>[2x]GPMDYYTLLGVDKGCSEDDLRRAYLKLAMKWHPDKHVNKGSKVEAEEKFKNICEAYSVLSDNEKRVKYDL

In the Laverania subgenus of malaria parasites, of which P. falciparum is the only human-infective member, a single Hsp70 chaperone, Hsp70-x, is exported to the host cell. Common to all Laverania parasites is an expanded set of exported proteins for host cell remodeling; thus, it is believed that Hsp70-x ensures the correct folding of these proteins, thereby supporting parasite survival and virulence functions. In addition to PfEMP1 and PfHsp70-x, J-dots contain multiple Hsp40 (also known as DnaJ) cochaperone proteins, which can stimulate Hsp70 activity. At least one of these cochaperones, PFA0660w (pf3d7_0113700), was shown to preferentially stimulate PfHsp70-x activity compared with a human Hsp70 (19).

Consistent with previous studies using full-length PFA0660w, the J-domain of this protein (PFA0660wJ) stimulated PfHsp70-x activity by ∼2-fold. We sought to investigate the structural basis of PfHsp70-x and Hsc70 stimulation by parasite cochaperones, focusing particularly on PFA0660w whose expression coincides with large-scale erythrocyte remodeling. To that end, we resolved the crystallographic structure of PFA0660wJ at 1.38 Å resolution and assigned the NMR spectra of PFA0660wJ in a sequence-specific manner. This allowed us to study the physical interaction of PFA0660wJ with PfHsp70-x or Hsc70 at amino acid–level resolution. As anticipated from the chaperone stimulation assays above, both PfHsp70-x and Hsc70 interacted directly with PFA0660wJ, as evidenced by changes in the intensity of [15N]-labeled PFA0660wJ NMR peaks corresponding to specific amino acids upon titration of this protein with unlabeled PfHsp70-x or Hsc70. Furthermore, we noted that PfHsp70-x produced larger changes in NMR peak intensity compared with Hsc70, suggesting that the PfHsp70-x–PFA0660wJ interaction is stronger than that between PFA0660wJ and the human chaperone, which is consistent with the biochemical assays above. To evaluate whether these interactions are compatible with the formation of canonical chaperone-cochaperone complexes, we mapped the PFA0660wJ amino acids showing the largest changes in NMR assays upon complex formation to the cochaperone domain structure; these amino acids are expected to define the direct protein binding interface. Both the PfHsp70-x and Hsc70 interactions primarily involved residues of the PFA0660wJ α-helix 2 (α2) forming a continuous binding surface toward the C terminus of that helix. Notably, these residues included PFA0660w H110, which is part of a conserved HPD motif found in Hsp40 cochaperones that is necessary for stimulation of Hsp70 activity.>[2x]MAHHHHHHVGTFENITAAPADPILGLADLFRADERPGKINLGIGVYKDETGKTPVLTSVKKAEQYLLENETTK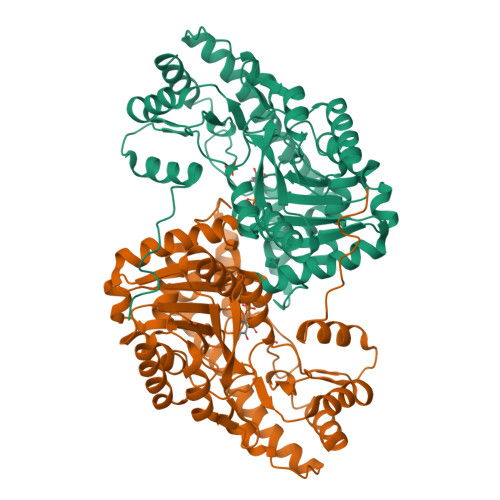NYLGIDGIPEFGRCTQELLFGKGSALINDKRARTAQTPGGTGALRVAADFLAKNTSVKRVWVSNPSWPNHKSVFNSAGLEVREYAYYDAENHTLDFDALINSLNEAQAGDVVLFHGCCHNPTGIDPTLEQWQTLAQLSVEKGWLPLFDFAYQGFARGLEEDAEGLRAFAAMHKELIVASSYSKNFGLYNERVGACTLVAADSETVDRAFSQMKAAIRANYSNPPAHGASVVATILSNDALRAIWEQELTDMRQRIQRMRQLFVNTLQEKGANRDFSFIIKQNGMFSFSGLTKEQVLRLREEFGVYAVASGRVNVAGMTPDNMAPLCEAIVAVL> GPAMKRARSANIPGAILHSLAELQDGLNAMIDPSWRAVRSLDNWALAITMESTELLDSYPWKWWKNLNATPDLANVRIELVDIFHFSLSGAMQMRSTPDDEIPAASLKPLKEVMTTFLPAKECTSDPYGFVFFPLTDTQNAIASFRNIIQLANAYRFDVIIECIIYAAEDLGFNLVAYYIAKHTLNCIRQLSGYKDGSYVKVNNGVEDN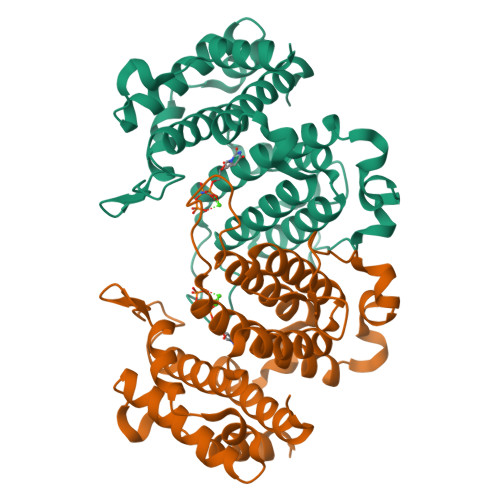SLLHNCIKDVSLDEVLDADKYVQAWNSIMANVYEAFQIKESDRKDAERWFALAKENRLAIKA>MGSSHHHHHHSQDPMSSLKYRLVTRSDFDGLVCAVLLKSIELIDDIQFVHPKDMQDGKVPITERDIITNLPYVANAHLVFDHHHSETLRNKGERPNHIINPNAPSAARVVWEHYGGTKTFPFEWVEMMEAVDKGDSAQFTRDEVLDSTGWNLLNFLMDARTGLGRFHNFRISNYNLMMALIDHCTHASIDEILQLPDVKERVELYRKHETLFKEQIQRCGKVYQNLVLLDLTEEETIYAGNRF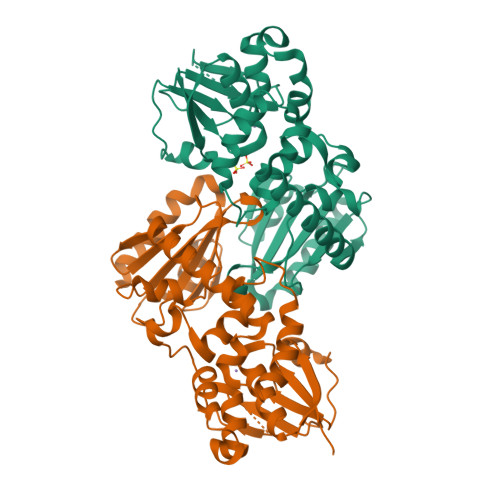IIYALYPQCNISIHKMWGFQKQNIVFATGKSIFDRSSRTNIGELMLKYGGGGHAAAGTCQIAIEDADRVEKALITQINADG[2x]> MLEQMISSSKVGVKINEWYKYIRLFSVPDSEILKAEVEEEIRHMKEDHDLLLYYSLMCFRHQLMLDYLEPKTLNEERPKISDLLEKIESSQTDLKGILEYYFNFFRGMYEFEQYEYLNAISFYKQAERKLSLVADEIERAEFHYKVAEIYYHMKQTHMSMHHIVQAIDSYKAHENYTVRVIQCSFVIGLNYLDMDYPEKAIPHFKNALDKAREIDMSRLIGSSLYNLGLCSFAEEAYEKASEYFKEGIRVYQDNGYEHSNRILDILLMLTKTTFKMRNHSEGISWCAHGLSLSKNLNDEIMAKMFEFIHALYVDNDNEKLNSILNYLELKSMLSDVEDLASDAAKYYNEKEDHKVAVAYYEKVLYARKQIQRGDCLYET;> RRGHTA

Proteins of the RRNPPA family are the most frequent pheromone receptors in Bacillota and use small secreted oligopeptides as pheromones. While most members of the RRNPPA family act as transcriptional factors through DNA binding, Rap receptors are specialized members that exhibit the capability to develop their function by interaction with specific protein targets. Binding of the pheromone produced from the propeptide, which is named Phr in this RRNPPA subfamily, induces Rap receptor inhibition. Our results reveal that distinct maturation processes generate multiple mature pheromones, which bind to receptors with varying affinities but produce identical structural and biological responses.

Initially, the structure of Rap3T was solved in complex with RRGHTA, the peptide with higher affinity and stabilization. The Rap3T-RRGHTA complex crystallized in C2221 space group, showing a monomer in the asymmetric unit, which generates by crystallographic symmetry the prototypical dimer observed in other crystal structures of Rap proteins. The structure revealed similar architecture to other Rap receptors, with an N-terminal 3-Helix bundle (3HB) domain (residues 1–69), followed by 7 tetratricopeptide repetitions (residues 95–376) conforming the TPR peptide-binding domain, connected by a linker of 26 amino acids (residues 70–94). The putative dimerization of Rap3T is due to the interaction of the 2 TRP domains that hide a large surface of TPR7 from the solvent. This surface is generated by the mutual interaction of the TPR7 and other TPR elements that conform the peptide-binding domain, explaining the cooperative effect observed in pheromone binding. All 4 peptides bind to Rap3T in the low nM range, but the internal Phr3T pheromone has the highest affinity (EC50 = 5,28 nM). As could be anticipated since all the structures show identical conformation, the analysis the Rap3T-peptide complex revealed a quite similar peptide recognition for all of them, with a core amino acid set critical for binding across all peptide versions. This core comprised N226, a conserved asparagine residue in Rap proteins that anchors the main-chain peptide and up to 23 other amino acids interacting with both pheromone side- and main-chain. Among this set of residues highlight the role of tyrosines Y151 and Y225 with several contacts with peptide residues in positions from 1 to 5, or D338 and Q182 that interact with the N- and C-terminal peptide ends. Comparison of complexes with RRGHTA and SRGHTS peptides showed that the sidechain of Arg in position 1 for RRGHTA mediates a network of salt-bridges with D264 and D335 plus hydrophobic interactions with M304 meanwhile the Ser in this position for SRGHTS only makes a hydrogen bound with Y225.sorbitol 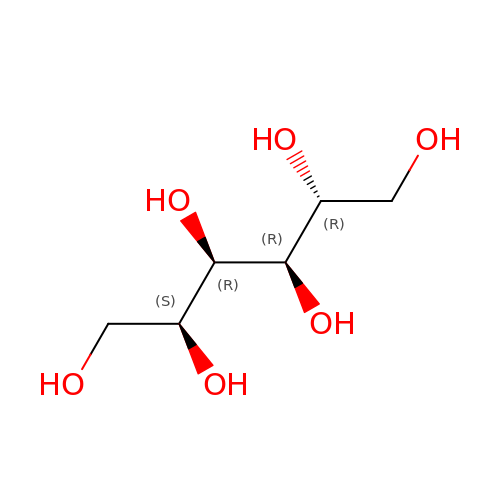| C6 H14 O6 | FBPFZTCFMRRESA-JGWLITMVSA-N>[4x]MAHHHHHHMTQRKGIILAGGSGTRLHPATLAISKQLLPVYDKPMIYYPLSTLMLAGMRDVLVISTPQDTPRFQQ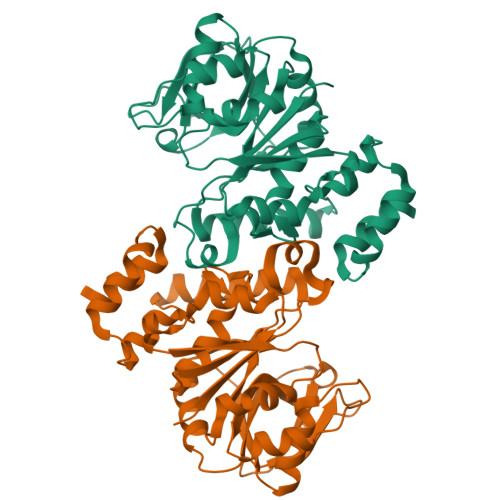LLGDGSQWGMNLQYAVQPSPDGLAQAFIIGEQFIGNAPSALVLGDNIYYGHDFQPLLKAADAQSSGATVFAYHVHDPERYGVVQFNAQGQAVSIEEKPKAPKSNYAVTGLYFYDQQVVDIAKAVKPSARGELEITSVNQAYMQQGQLNVQTMGRGYAWLDTGTHDSLLDASQFIATLENRQGLKVACPEEIAWRSGWINASQLEALVQPLTKNGYGQYLMQILKETVF> MAKENTQQKEIKRQPAVELAVFNLNSVTDVADLQMIASQVQLYLQVCGNTTLEQIKSKANITTVANIFALTGSVLDLMLYATDKKTGDAAVQRGALLAANLIGLFSEPNNEAHARMALRPMFGLMAECLYRENGKIKETDIKRLGLHLNAMIAGDLENFLKETQAKLSSLLISATTLGVTILQSMATPATGINAGITTAAGASAEKRDPKLKFTNWAVPLIDLLGKPSQANLTPKIQPNITSRLQQEATQAIAALSQTLQQQANAGQKYTLAWLLQETLKAIQALENKGNASVPINQTGEYERHTKGDTLEFVSLQADALNAPPCEGADSQSGKSISYSIGAERVQHADFYLPKIGFSFIRQYNSQMDEFDQSMVGARWMMPFSNMIQQNAQGYLFIDSKGRKHQLPVSIIFETYEVPYEGWIIKPLKNGELILDFGGEWRSHFQSFDGGKNYYLVKKMNETSQEEILLEYLLLDHIAYLKVINFKLKQAEYELKFAFNEQVKIIAVFLDDKAEPLARYEYDTQGNLIKAIDQNGHTRTYEYNQFHQLTRYTDRTGRGQNIRYESTEAKAKAIEEWADDGSFHTKLKWHPRLRQVAVYDAYDVPTYYYFDLDGFTYRTRLADGRESWYSRDGKKRITRQIDFDGRETQQEYNDQDQLVKIVQPNGGIIRFAYNKQGNLVEIKDPEGSIWKREYDENRNVSKEINPLGHITQYKYNNDNQLVEVIDAKGGVKKIQYNELGQMISYTDCSGKSSTWEYDEDGALTAEQTANNKVVQYFYSTKGRDKGQLQSIIYPDGLKEYFEHDEEGRLLKHTDTKGLVTEYKYNQVGLLEQRIDANRHSVAYQWDKQGRIQKLINQNQAEYLFGYNPYGYLIREQAFDGEEKHYSYNENGRLFQIRRPNILTQFDYYADGQIASKSFTHLHTGQKQTEQFDYNLNSQLSRASNEVSQIDLYRNALGQLVREHQHYKIPELKPLTAVLHYEYDELGNLIKTIRPDGHTLNHLVYGSGHIYAIGLNNQEVVSFQRDDLHRETTRLLANGLMQTKQYNDVGLLSSQFIQPEQETQDYLQYQAHRKYHYDKNYLLSQVEDSRLGKLNYQYDPIGRLIAAQSLHKTESFNFDPAGNLIDSESVLSPAQIKNNLIKSYKGKHYQYDVQGNVTEIIQAGKNLKLTWDNQNRLIRSDNNGLVTEYGYDVFGRRLYKKTAKELTLFGWDGDLMIWESFKSAQTNYTKHYIYEPDSFVPLLQAGYKDFIQLIETPDYQEYQTKPYSIYKDPVWNRNLGKERTALEQFTFYHCDQVGTPQTMTNIRGECVWEILQDTWGAVSQIKALNQDNPFEQNNLRFQGQYYDRETELHYNRYRYYEPHSARYVSKNPIGLEGGMNTSSYVSDPNQWINPKGLNSFNYGEMFGIPASAQSGLAYQGQRNYECYAETGELCKIKVPPLFDYVACSGGGLGIGVGFVKNQWTGEYYISGSKDSLLIPVAKSVAQNKQFSAKDLAGASCVGGNIHNIPSYTKTTMTMGEITNEFVSGASVTVGGGAYGAVANVVVPLVSKSSPVKGTWASELGVGTPGFNVGVSGTVSVDTILDAVKPSKKHHHHHH

The type VI secretion system (T6SS) is a molecular machine utilised by many Gram-negative bacteria to deliver antibacterial toxins into adjacent cells. Here we present the structure of Tse15, a T6SS Rhs effector from the nosocomial pathogen Acinetobacter baumannii. Tse15 forms a triple layered β-cocoon Rhs domain with an N-terminal α-helical clade domain and an unfolded C-terminal toxin domain inside the Rhs cage. Tse15 is cleaved into three domains, through independent auto-cleavage events involving aspartyl protease activity for toxin self-cleavage and a nucleophilic glutamic acid for N-terminal clade cleavage.

We mutated the equivalent two aspartic acid residues (D1369N, D1391N) to asparagine in a single construct (Tse15NN). SDS-PAGE analysis of the purified Tse15NN showed only two protein fragments, compared to the three observed during purification of wildtype Tse15. Indeed, the 22 kDa toxin CTD observed in the Tse15 purification was absent in the Tse15NN purification and the Rhs domain fragment showed a corresponding increase in size. The identity of this toxin protein fragment was confirmed by mass spectrometry peptide fingerprinting, thus confirming that wildtype Tse15 possesses aspartyl protease activity that drives self-cleavage of the toxin from the Rhs domain. Unlike wildtype Tse15, particle processing for the cryo-EM data of Tse15NN showed only one main monomeric 3D particle class with the clade domain predicted to be retained together with the body of the Rhs cage. Tse15NN particles were compiled to produce a map to a maximum resolution of 1.77 Å and showed that the Tse15NN quaternary structure is the same as the wildtype (RMSD 0.860 Å over residues 14–1395, A chain). Clear, connective density was observed after L1395 and the sequence of the toxin could be mapped up to residue 1484, guided by a difference map as well as the unsharpened map. After residue 1484, significant breaks in connective density meant that the C-terminal of the toxin could not be placed into the maps. Overall, the position of the Tse15NN toxin was similar but not the same as the wildtype Tse15, and lacked defined secondary structure features. We also could not find equivalent density for the helix that was present in the Rhs domain opening but did show the toxin peptide was still in close proximity to the end of the clade domain.>MSEIGTGFPFDPHYVEVLGERMHYVDVGPRDGTPVLFLHGNPTSSYLWRNIIPHVAPSHRCIAPDLIGMGKSDKPDLDYFFDDHVRYLDAFIEALGLEEVVLVIHDWGSALGFHWAKRNPERVKGIACMEFIRPIPTWDEWPEFARELFQAFRTPDVGRELIIDQNAFIEGILPKFVVRPLTEVEMDHYREPFLKPVDREPLWRFPNELPIAGEPANIVALVEAYMNWLHQSPVPKLLFWGTPGVLIPPAEAARL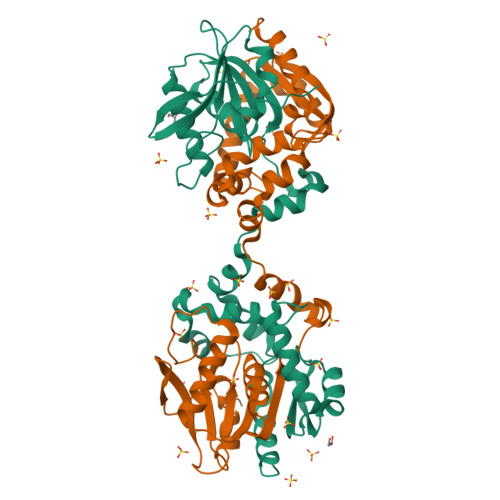AESLPNCKTVDIGPGLHYLQEDNPDLIGSEIARWLPALHHHHHH[4x]> TTHFVIIDRDGTVVSSTNTLSNFFGTGKYTAGFFLNNQLQNFGSEGFNSYEPGKRSRTFMAPTVLKKDGETIGIGSPGGNRIPQILTPILDKYTHGKGSLQDIINEY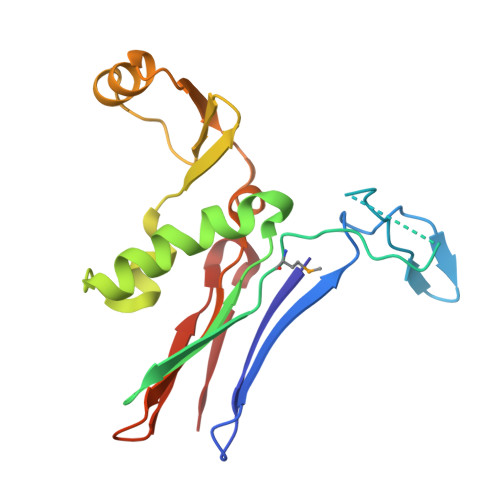RFTFEKNTAYTEIQLSSEVKNELSRKGLNVKKKVSPAFFGGVQALIKDERDNVITGAGDGRRNGTWKSNK>[2x]AEFQVTSNEIKTGEQLTTSHVFSGFGCEGGNTSPSLTWSGVPEGTKSFAVTVYDPDAPTGSGWWHWTVVNIPATVTYLP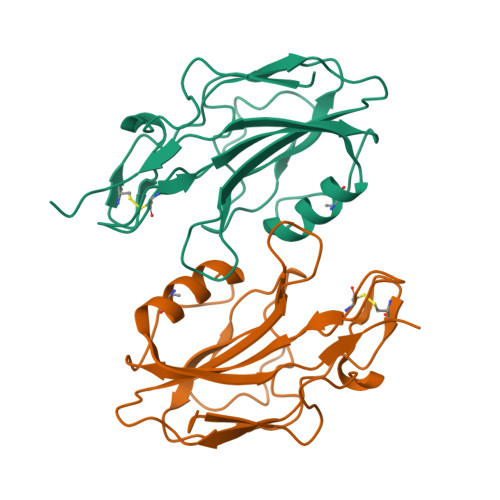VDAGRRDGTKLPTGAVQGRNDFGYAGFGGACPPKGDKPHHYQFKVWALKTEKIPVDSNSSGALVGYMLNANKIATAEITPVYEIKLE>GSGDQLKPVDALQCYDCHTQIEDMHVVGKHATVNCVHCHDATEHVETASARRMGERPVTHTSPEACASCHTAQFNSFASVRHESHPREEKANPRSRSPKFDTLIGAHGFSLEHAEPRSHAFMLVDHFIVDRAYGGRFQYKSWQNVTDGLGAVRGAWTVIEDMDPTTSDQRRFLAQTATAANPVCLNCKTQDHILDWAYMGDEHDAAKWARTSKVVDFARDLHHPVNCYMCHDPHSTEPRVVRDALIHAVVDQGLGTYPYDEAKSEHVTLTPVTFQRGGEDFRKIGLLNVADSNLMCGQCHVEYNCNPGFQQSDGAPVGMDDRRTNHFFWANVFDYAEAAKEIDFFDFTHVTTGAPLPKLQHPELETFWGSTHERNGV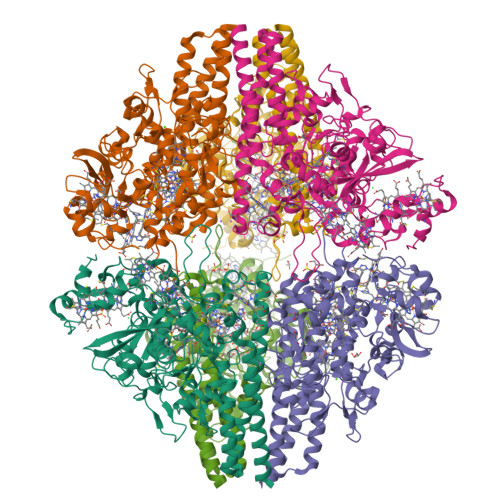TCADCHMPRVKLENGKEYTMHSPRTPRDMMNRACLNCHDGWTEAEAEYAIDYIKNYTHGKIMKAEFWLARMIDLFPVAKRAGVSEDVLNEVRALHYDAHLHWEWWTAENSVGFHNPDQARESLMKSITKSKEGVGKLDAAIDAAVAAN[2x]> ADPGMDEITITTQPKSGYVIRNKPLRLQCRANHATKIRYKCSSKWIDDSRIEKLIGTDSTSGVGYIDASVDISRIDVDTSGHVDAFQC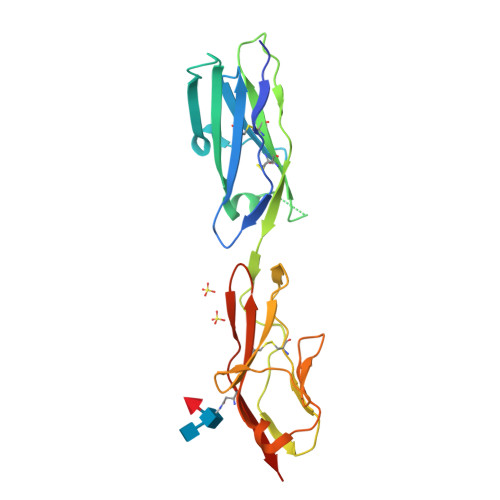QCYASGDDDQDVVASDVATVHLAYMRKHFLKSPVAQRVQEGTTLQLPCQAPESDPKAELTWYKDGVVVQPDANVIRASDGSLIMSAARLSDSGNYTCEATNVANSRKTDPVEVQIYHHHHHH>[2x]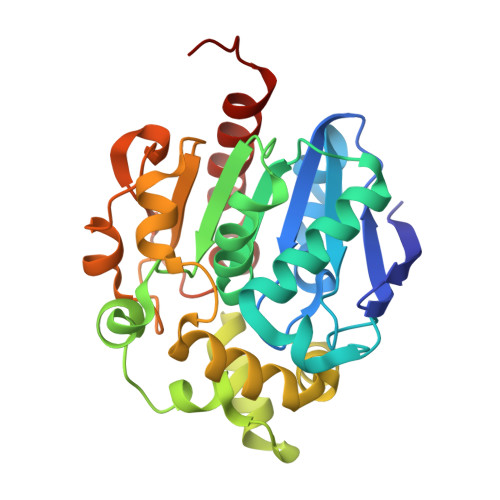MTINYHELETSHGRIAVRESEGEGAPLLMIHGNSSSGAIFAPQLEGEIGKKWRVIAPDLPGHGKSTDAIDPDRSYSMEGYADAMTEVMQQLGIADAVVFGWSLGGHIGIEMIARYPEMRGLMITGTPPVAREEVGQGFKSGPDMALAGQEIFSERDVESYARSTCGEPFEASLLDIVARTDGRARRIMFEKFGSGTGGNQRDIVAEAQLPIAVVNGRDEPFVELDFVSKVKFGNLWEGKTHVIDNAGHAPFREAPAEFDAYLARFIRDCTQLEHHHHHH>[6x]MGKACLQNGTRLLRADGSEVLVEDVQEGDQLLGPDGTSRTASKIVRGEERLYRIKTHEGLEDLVCTHNHILSMYKERFGREGAHSPSAGTSLTESHERVDVTVDDFVRLPQQEQQKYKLFRSTDFVRREQPSASKLATLLHINSIELEEEPTKWSGFVVDKDSLYLRYDYLVLHNS

At the heart of the spliceosome is pre-mRNA processing factor 8 (Prp8), a large (approximately 270 kDa) and highly conserved protein. Prp8 helps generate mature mRNA by coordinating critical rearrangements at the catalytic core of the spliceosome. The intein-containing precursor undergoes protein splicing, a process that excises the intein and ligates the flanking sequences, called exteins, to form the functional protein. The intein is also found at a highly conserved site at the center of Prp8 and thus is at the core of the spliceosome.

The Cne Prp8 intein was solved to 1.75 Å resolution. The Cne Prp8 intein structure represents only the second known fungal nuclear intein structure. As with all solved intein structures so far, the Cne Prp8 intein has the canonical horseshoe shape, created by pseudo–2-fold symmetry that positions the catalytic N- and C termini in close proximity. Highlighting the splicing blocks (A, B, F, and G), we see the active core that carries out autocatalytic protein splicing. This catalytic center contains the residues essential for splicing: the nucleophilic cysteine (C1) in Block A, and the terminal asparagine (N171) in Block G. The C1 and N171 are also positioned in the vicinity of the conserved Block B TxxH residues (T62 and H65), which are important for priming the intein for self-excision at its amino terminus. For example, Blocks A and B are far apart in sequence but fold proximally in 3D space to execute protein splicing. This representation also illustrates that the unresolved regions of the intein are between Block B and Block F and likely represent flexible linker sequences of a former endonuclease domain. The unstructured regions in the Cne Prp8 intein structure are where the Sce Vma1 intein encodes a linker domain (dashed red lines). A closer look at the active centers of the Cne Prp8 intein and the Sce Vma1 intein demonstrates unmistakable overlap of the catalytic residues, further confirming the similarities. The Cne Prp8 intein only has 2 cysteines: C1 in Block A, and C61 in Block B, immediately preceding the TxxH motif (blue arrowheads).>[3x]XEWEALEKKLAALESKCQALEKKLEA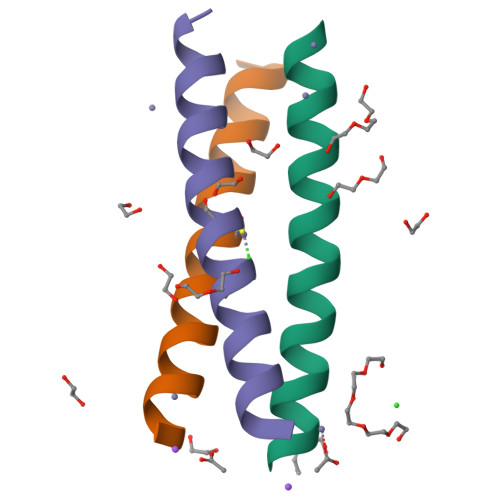LEHGX>[12x]SMAPGQSKKKIFKPEELRQALMPTLEALYRQDPESLPFRQPVDPQLLGIPDYFDIVKSPMDLSTIKRKLDTGQYQEPWQYVDDIWLMFNNAWLYNRKTSRVYKYCSKLSEVFEQ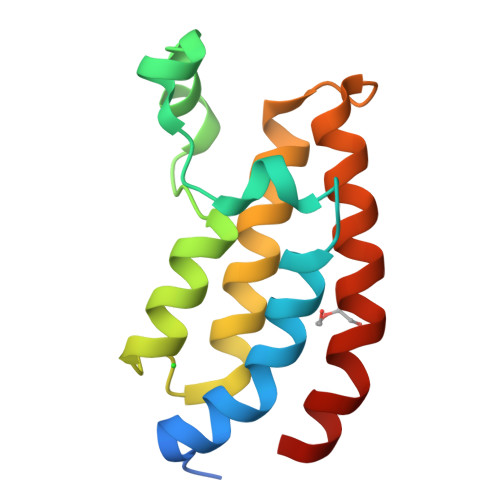EIDPVMQSLG> MDVQETQKGALKEIQAFIR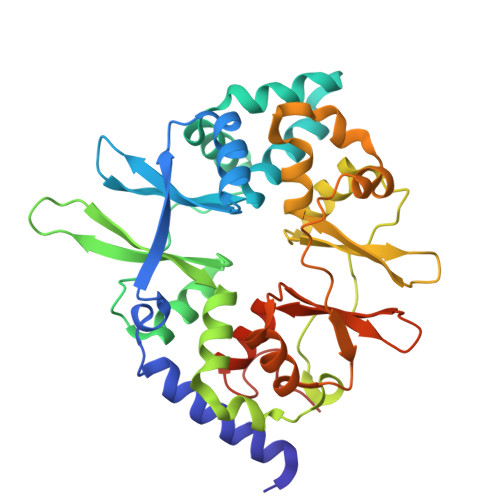SRTSYDVLPTSFRLIVFDVTLFVKTSLSLLTLNNIVSAPLWDSEANKFAGLLTMADFVNVIKYYYQSSSFPEAIAEIDKFRLLGLREVERKIGAIPPETIYVHPMHSLMDACLAMSKSRARRIPLIDVDGETGSEMIVSVLTQYRILKFISMNCKETAMLRVPLNQMTIGTWSNLATASMETKVYDVIKMLAEKNISAVPIVNSEGTLLNVYESVDVMHLIQDGDYSNLDLSVGEALLKRPANFDGVHTCRATDRLDGIFDAIKHSRVHRLFVVDENLKLEGILSLADILNYIIYDKTTTPGVPEQTDNFESAV{[2-(6-AMINO-9H-PURIN-9-YL)ETHOXY]METHYL}PHOSPHONIC 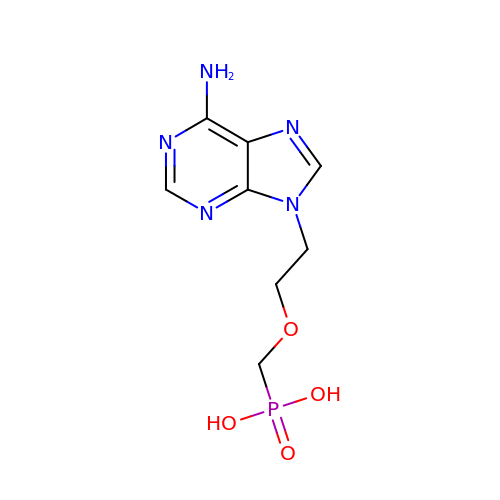ACID | C8 H12 N5 O4 P | SUPKOOSCJHTBAH-UHFFFAOYSA-N> MVKEIHVEGFEAYSKAAEENNGKNIFALFCGSKDANGESWCPDCVTAEPVIARNLKYAPADSVFIHCSVGERAFWKDQSNVFRKDPVL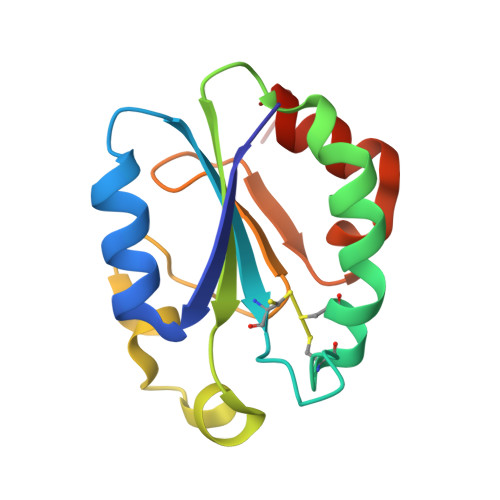KLKCVPTLLKPGTPQRLEEEQCADDNLVQMFFQEELEHH>[2x]GSGEIRPTIGQQMETGDQRFGDLVFRQLAPNVWQHTSYLDMPGFGAVASNGLIVRDGGRVLVVDTAWTDDQTAQILNWIKQEINLPVALAVVTHAHQDKMGGMDALHAAGIATYANAL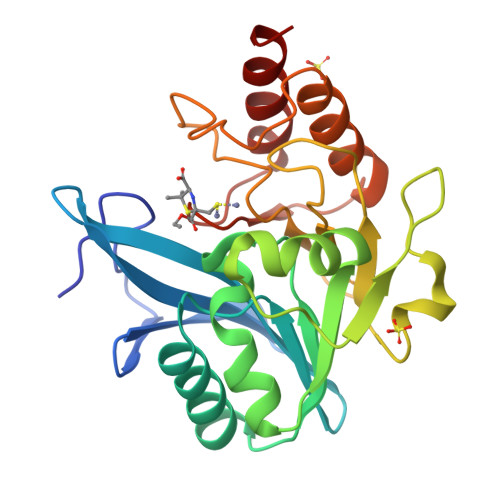SNQLAPQEGMVAAQHSLTFAANGWVEPATAPNFGPLKVFYPGPGHTSDNITVGIDGTDIAFGGCLIKDSKAKSLGNLGDADTEHYAASARAFGAAFPKASMIVMSHSAPDSRAAITHTARMADKLR>[2x]MADTKAKLTLNGDTAVELDVLKGTLGQDVI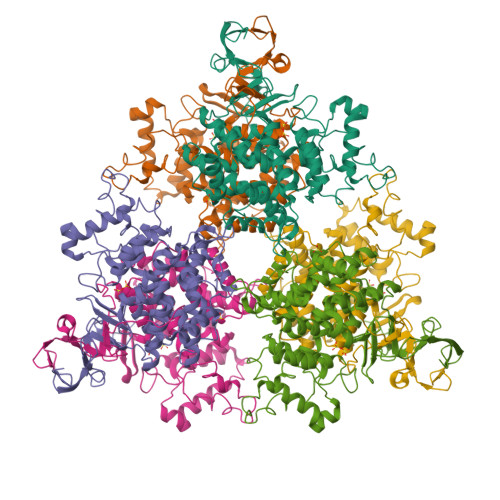DIRTLGSKGVFTFDPGFTSTASCESKITFIDGDEGILLHRGFPIDQLATDSNYLEVCYILLNGEKPTQEQYDEFKTTVTRHTMIHEQITRLFHAFRRDSHPMAVMCGITGALAAFYHDSLDVNNPRHREIAAFRLLSKMPTMAAMCYKYSIGQPFVYPRNDLSYAGNFLNMMFSTPCEPYEVNPILERAMDRILILHADHEQNASTSTVRTAGSSGANPFACIAAGIASLWGPAHGGANEAALKMLEEISSVKHIPEFFRRAKDKNDSFRLMGFGHRVYKNYDPRATVMRETCHEVLKELGTKDDLLEVAMELENIALNDPYFIEKKLYPNVDFYSGIILKAMGIPSSMFTVIAAMARTVGWIAHWSEMHSDGMKIARPRQLYTGYEKRDFKSDIKR>TEEKTCDLVGEKGKESEKELALLKRLTPLFQKSFESTVGQSPDMYSYVFRVCREAGQHSSGAGLVQIQKSNGKETVVGRFNETQIFQGSNWIMLIYKGGDEYDNHCGREQRRAVVMISCNRHTLADNF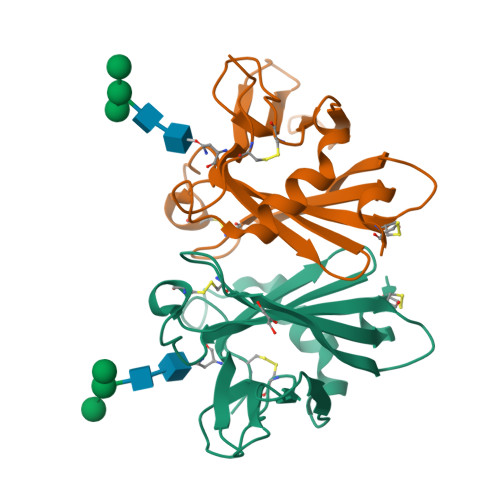NPVSEERGKVQDCFYLFEMDSSLACS[2x]> MAEHEQVNWPYVNTKLKRDPAVEAQIEKLLAKMTIEQKVAQMIQPEIGYLTVEQMRKYGFGSYLNGGNTAPYGNKRADQATWLKYADEMYLAAMDSTLDGIAIPTVWGTDAMHGHSNVYGATLFPHNIGLGAARDTDLIKRIGQATAKEVAATGIEWSFAPTVAVVRDDRWGRTYESYSEDPDLVKRYAGEMVTGIQGDVGADFLKGSNRIATAKHFVGDGGTERGVDRGNTLIDEKGLRDIHSAGYFSAINQGVQSVMASFNSWNGKRVHGDKHLLTDVLKNQLGFDGFVVSDWNAHKFVEG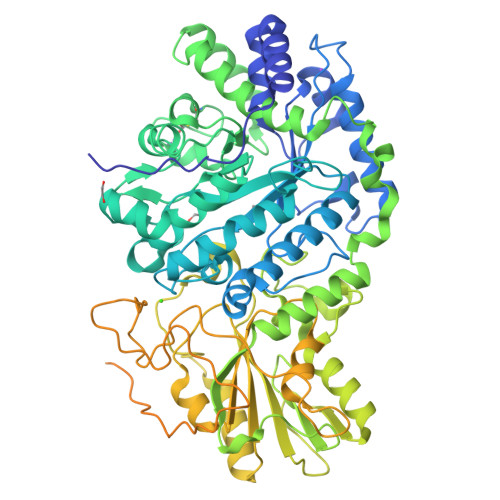CDLEQCAQAINAGVDVIMVPEHFEAFYHNTVKQVKAGVIAESRINDAVRRFLRAKIRWGVFTKSKPSARPESQHPQWLGAAEHRTLAREAVRKSLVLLKNNESILPIKASSRILVAGKGANAINMQAGGWSVSWQGTDNTNSDFPNATSIFSGLQSQVTKAGGKITLSESGEYTSKPDVAIVVIGEEPYAEWFGDIELLEFQHETKHALALLKQLKADNIPVVTVFLSGRPLWVNKELNASDAFVAAWLPGSEGEGVADVLLTNKQGKTQFDFTGKLSFSWPKYDDQFTLNLNDADYDPLFAYGYGLTYQDNINVPVLSEKTSPKKTVNSDSHPLFVRSLAKNMTWQLADTSTQKVLASGASATSGDKQSLLMQSVNLSYQEDGRGFNWRAQAALSLSYLEPTPLDSKFSTGYLELKMRIDKAPEQGANLQVMCSESNCLRDIDFSSFSQLMADKSWHTLAIPLHCDDSDQAEQPITDALRITSQNLSLAIADVALTIKPSDDSISLTCAKLEHHHHHH> XWAREIGAXLR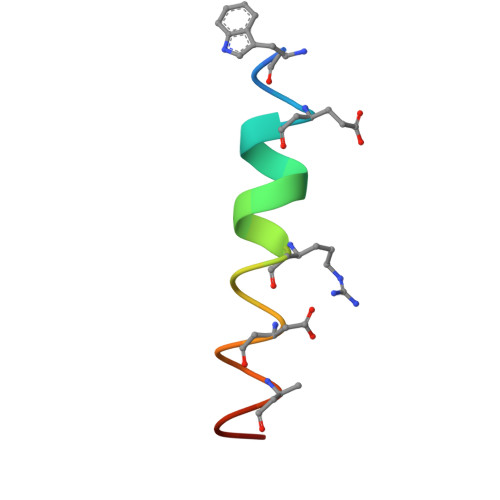RMADDLNAQYEX> LDKVYQMKSKPRGYCLIINNHNFAKAREKVPKLHSIRDRNGTHLDA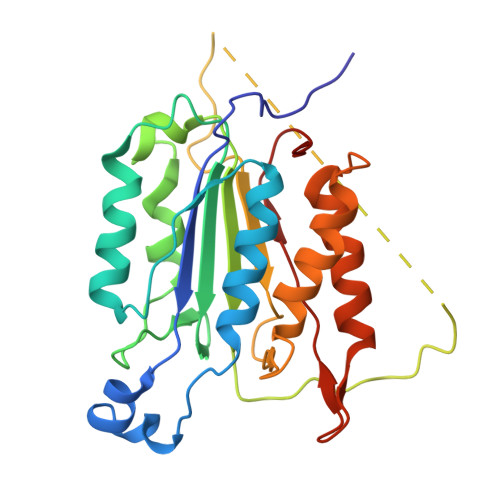GALTTTFEELHFEIKPHHDCTVEQIYEILKIYQLMDHSNMDCFICCILSHGDKGIIYGTDGQEAPIYELTSQFTGLKCPSLAGKPKVFFIQACQGDNYQKGIPVETDSEEQPYLEMDLSSPQTRYIPDEADFLLGMATVNNCVSYRNPAEGTWYIQSLCQSLRERCPRGDDILTILTEVNYEVSNKDDKKNMGKQMPQPTFTLRKKLVFPSD> MQQRKKIYLRQKRKIYIQLKNKEKKKNNQFIQKREKMGYKIRNKSIFWTRAGWKNNWHPKNFNAPRPSYGEFTMGIRCRNDHHSFLRYVQTYRNMSRHCKQYFLGDKQLEETFILGLRSLFLVPYDSQCLTDQIKHGGERRFVDQLDRDFELISYNTHPYQLFTYTVRNEHLAWKNEQYEKIQKGEKTFEQELLDYLDEQVLAEKAKLRDGQNFSIERMT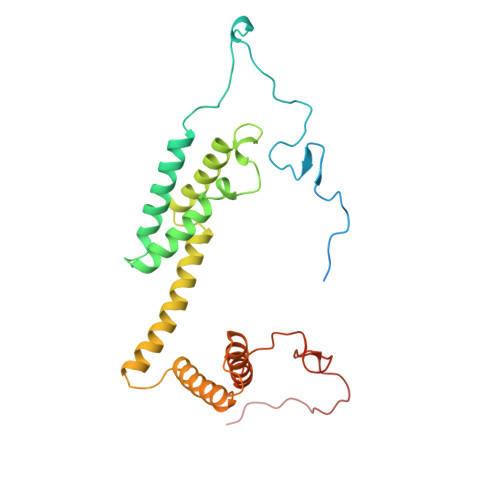EIALHVFRKARAGKVRPAQDVRGPDGNVNDFLEQRRPFEHPNPTGVTH>[2x]SDLPMPMRFRHLKKTSKEAVGVYRSPIHGRGLFCKRNIDAGEMVIEYAGIVIRSILTDK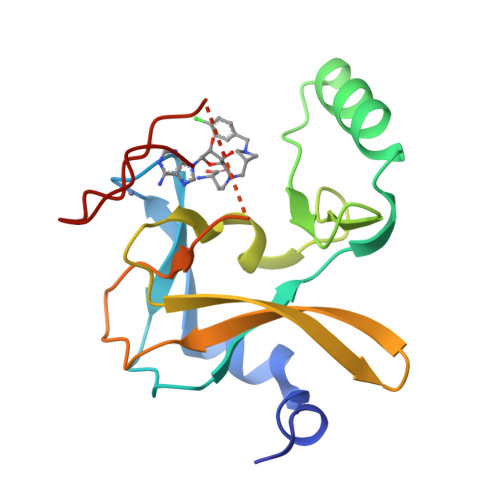REKYYDSKGIGCYMFRIDDSEVVDATMHGNAARFINHSCEPNCYSRVINIDGQKHIVIFAMRKIYRGEELTYDYKFPIEDASNKLPCNCGAKKCRKFLN> MFSLTQTWLIAHWYCGHKFRHRFMRDKRFHPSLQAS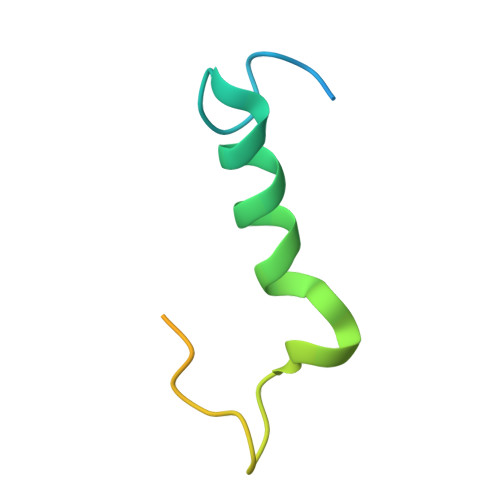HDARNRFSKRRHFKTNRWNYQQAYRDMP>GSHMGQKNTTKEETTEPADTDKRIEAPTFNADSAYAYIERQVAFGPRVPNTEAHQRCADYLAGELDRHGAKVYVQEAVLTAYNGEKLKAQNIVGAFQPEKSRRVLLFAHWDSRPYADHDTDEANHRKPIDGADDGGSGVGILLEIARQIQAKAPAIGIDIVFFDAEDYGTPEFVDEYKPDTWCLGSQFWAKNPHVPNYKAEFGILLDMVGSRGATFYKESTSVQYAARYVEKVWTAARELGYGKYFINAQGGAIVDDHQYVIQGLRTPCLDIINY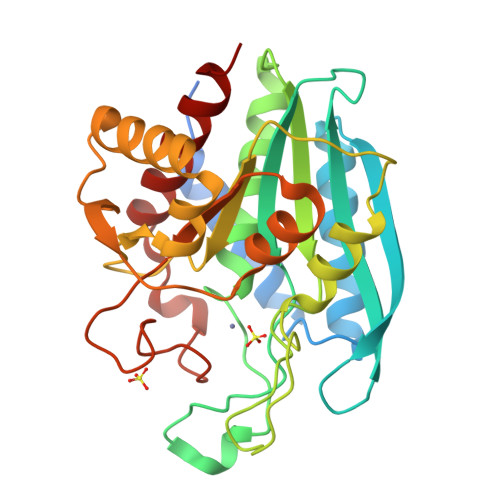DPDTQSGFGPYWHTQNDTMENIDRETLKAVGETILNVIYNEK[4x]>[4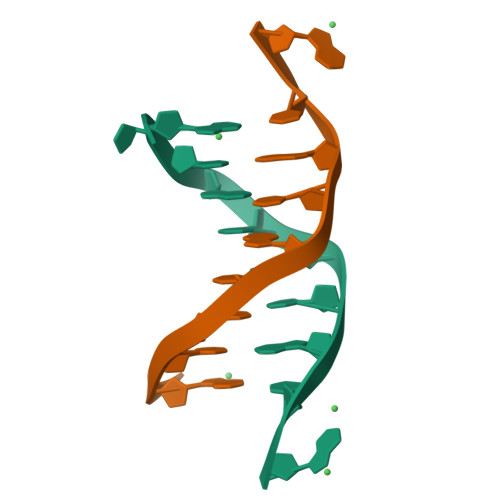x]CGTGTACACG>VGPIQSIKVDPMKSGGLGVVYRSPDKGRVSLYLYNDGEDILLVVDARFDWRGEQNVLVLNSKFAGGEWGPEVRPEGFPFPCCGYVTTITVRVEIGADGFTLSANGIEIVKYPYRDGLPPP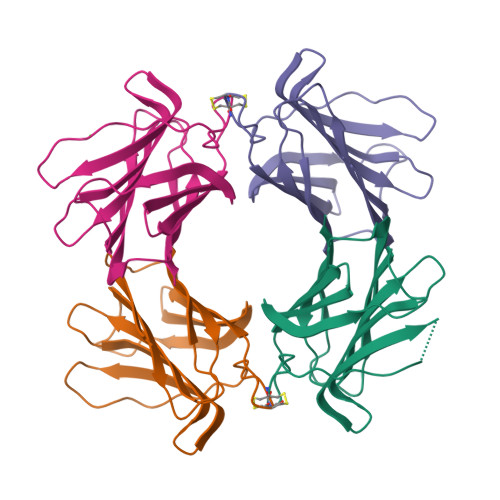VTKFQYVFQDQGASETAQLESLSAYY[4x]>[3x]MRTTKFLALA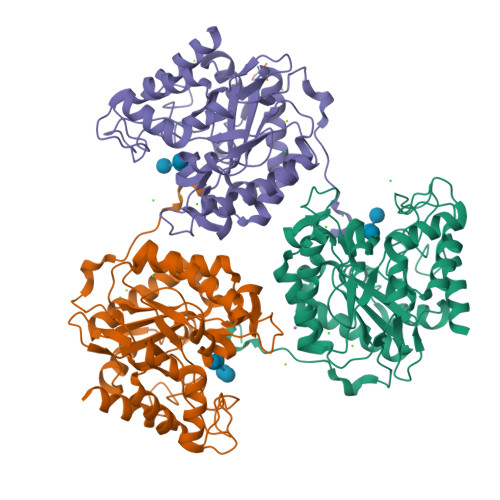LCLLASASALSANNSAPSNDWWDIPYPSQFDVKSLKTQSFISVKGNKFIDDKGKTFTFRGVNIADTGKLLSRNQWQKSLFEELANNWGVNTIRLPIHPVSWRKLGPDVYLGHIDEAVRWANDLGIYLILDWHSIGYLPTEQYQHPMYDTTIKETRDFWRRITFRYQNVPTVAVYELFNEPTTMGNTLGERNWAEWKTLNESLIDMIYASDKTVIPLVAGFNWAYDLSPIKKAPIEREGIAYAAHPYPQKAKPEVKNDKNFFKLWDEKWGFAADTYPVIATQLGWVQPDGYGAHIPVKDDGSYGPRIVKYMQKKGVSYTVWVFDPDWSPTMINDWDFTPSEQGAFFKQVMLEAKKR(phenylmethyl)azanium | C7 H10 N | 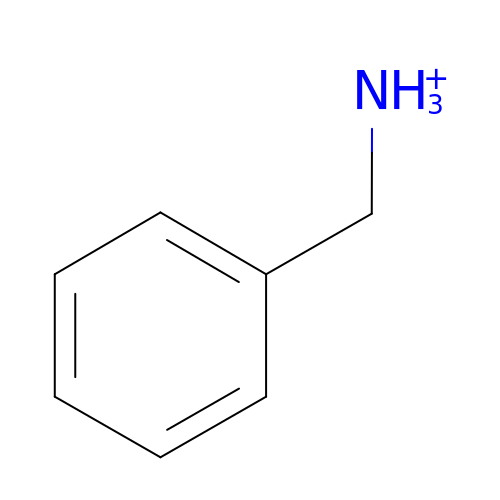WGQKYBSKWIADBV-UHFFFAOYSA-O> MVAQFQIECVESNT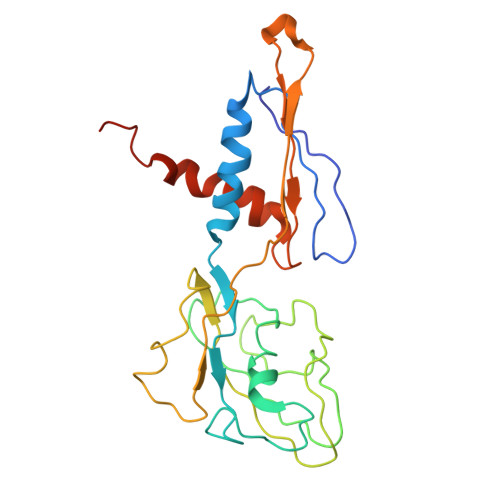EESRNHYSKFILEPLERGQGTTVGNALRRVLLSNLEGTAVTAVRIAGVSHEFATVPGVREDVLEIIMRMKEVILKSYSSQAQIGRLLVNGPTTITASHFDLPSEVEVIDPTQYVATIAEGGKLEMEFRIERGKGYRTVERGREEATSLDFLQIDSIFMPVRKVNYSVEEVRADGSIPKDRLLLEVWTNGSISPQEALSSAAGILVDLFNPLKDISLEPTDTN> MDEKSTKIIMWLKKMFGDKPLPPYEVNTRTMEILYQLAEWNEARDKDLSLVTEDLKLKSAEVKAEAKYLQDLLTEGLGPSYTN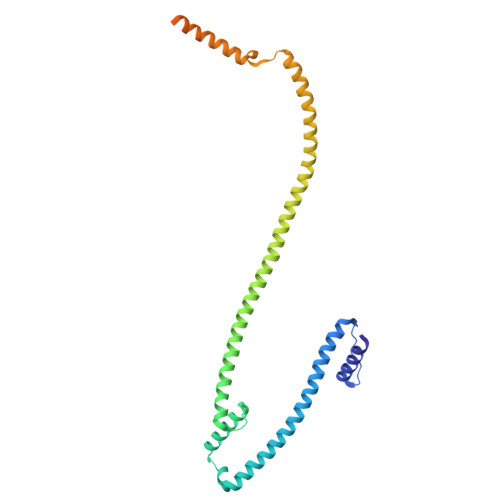LSRMGNNYLNQIVDSCLALELKNSSLSSYIPAVNDLSSELVAIELNNQEMEAELTSLRKKLTEALVLEKSLERDLKKAEEQCNFEKAKVEIRSQNMKKLKDKSEEYKYKIHAAKDQLSSAGMEEPLTHRSLVSLSETLTELKAQSMAAKEKLNSYLDLAPNPSLVKVKIEEAKRELKATEVELTTKVNMMEFVVPEPSKRRLK> PISPIETVPVKLKPGMDGPKVKQWPLTEEKIKALVEICTEMEKEGKISKIGPENPYNTPVFAIKKKDSTKWRKLVDFRELNKRTQDFWEVQLGIPHPAGLKKKKSVTVLDVGDAYFSVPLDEDFRKYTAFTIPSINNETPGIRYQYNVLPQGWKGSPAISQSSMTKILEPFKKQNPDIVIYQYMDDLYVGSDLEIGQHRTKIEELRQHLLRWGLTTPDKKHQKEPPFLWMGYELHPDKWTVQPIVLPEKDSWTVNDIQKLVGKLNWASQIYPGIKVRQLSKLLRGTKALTEVIPLTEEAELELAENREILKEPVHGVYYDPSKDLIAEIQKQGQGQWTYQIYQEPFKNLKTGKYARMRGAHTNDVKQLTEAVQKITTESIVIWGKTPKFKLPIQKETWETWWTEYWQATWIPEWEFVNTPPLVKLWYQLEKEPIVGAETFYVDGAANRETKLGKAGYVTNKGRQKVVPLTNTTNQKTELQAIYLAL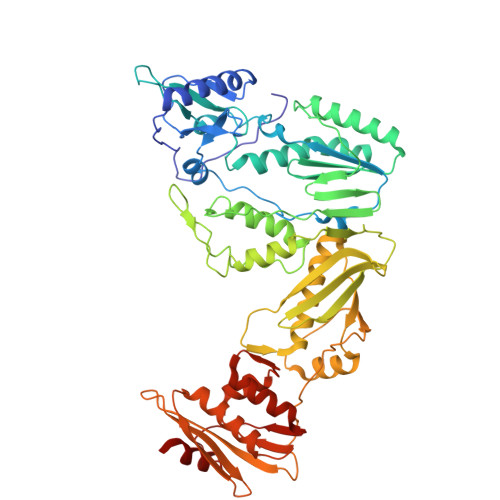QDSGLEVNIVTDSQYALGIIQAQPDKSESELVNQIIEQLIKKEKVYLAWVPAHKGIGGNEQVDKLVSAG>[12x]MESTFIMIKPDGVQRGLIGEIISRFEKKGFYLKALKLVNVERSFAEKHYADLASKPFFQGLVDYIISGPVVAMVWEGKSVVTTGRKIIGAT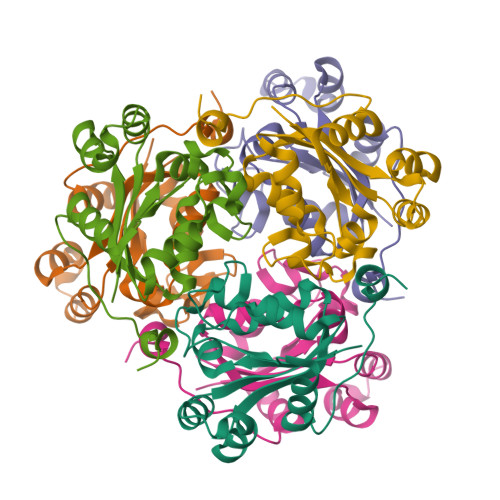NPLASEPGTIRGDFAVDIGRNVIHGSDSIESANKEIALWFPEGLADWQSSQHPWIYEK>MVLYFIGLGLYDERDITVKGLEIAKKCDYVFAEFYTSLMAGTTLGRIQKLIGKEIRVLSREDVELNFENIVLPLAKENDVAFLTPGDPLVATTHAELRIRAKRAGVESYVIHAPSIYSAVGITGLHIYKFGKSATVAYPEGNWFPTMYYDVIKENAERGLHTLLFLDIKAEKRMYMTANEAMELLLKVEDMKKGGVFTDDTLVVVLARAGSLNPTIRAGYVKDLIREDFGDPPHILIVPGKLHIVEAEYLVEIAGAPREILRVNV[2x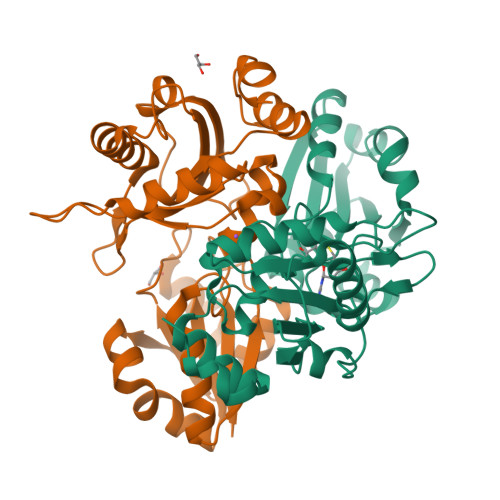]> GPMSVPTDGAVTTSQIPASEQETLVRPKPLLLKLLKSVGAQKDTYTMKEVLFYLGQYIMTKRLYD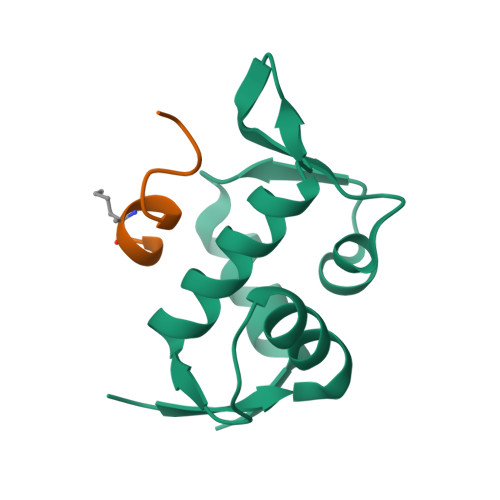EKQQHIVYCSNDLLGDLFGVPSFSVKEHRKIYTMIYRNLVVVNQQESSDSGTSVSEN> SGSKYVVIDGEGNEYEFTDLKEAAAKAKELKKKYGFASISVPVEPDEVAVVDGKGNEHTFTDIKKAVEKAK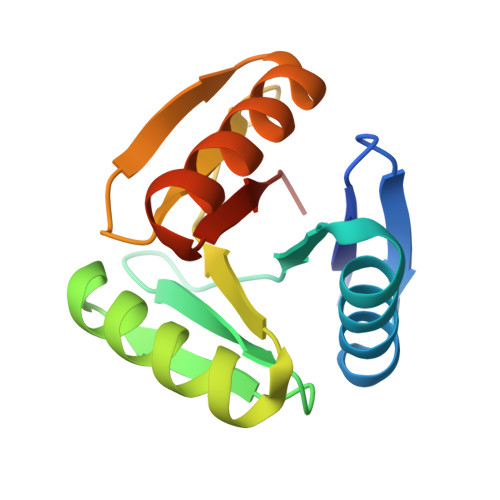ELAKETGFASISVPVEPDEYLVIDGKGNEHKFTDLKEAVAKAKELKKKYGFASVSVPVPAGSG>GAMGEQIFYWSPAKHWRMSDEGVVIGESTYTGMILEWFPEFYFFAQTGVTINRLLERFSSGSEKEANEILELLIQDRVLVEGILPPREVFSPQEGLFVNPYSEQIRYSKEALDYYVSEQLNRTHAACRSTKIQLETSGALPDIIQKRRSCRRFDMKTPVSFATFSNLLSSLKQRKEDKILYNYASAGGLYPIDVFVYVKPRRVEGVKAGFYYFNPADHSLVLVNNIDQVIKDDHELINQDIFAQSAFSVYLVYNARASMPKYGAAGYFYACIEAGIITATLNMVAEDLNVGLCSIGHMNFEEIQTFLKLEDHQVILHAIEGGLKIDGAAAENLYFQ[2x];> GAMEADLSEPFSLTEVQTAYMLGRNPQFELSGISPQTYFEYETELDIARLSRSFQKVIQRHPMLRAVILPEGKQQILRDVPEYEIEVESLVSMPPEKQAARLREERSRMIDHVFPLGQWPLFELKAFQLQEHTYLLCFRYDALLMDGASMNLVGQDLMHYYHQPDAQLPPLSFTFQDYMHIYDDMKRGTEYETAKAYWTNKLPDFPPAPSLLLAKDPAEIGTPNFQSLTTIITKDKWLKLRRLAQDKQVTPSALLCTVYGEVLAFWSNQRRLAINLTVFNRYPVHDEVEQIVGDFTSLILLDMDMDQKQPFFTKVEQTQSTLLDGLEHRHYDGVEFIRDYTRYHQMRPKAVMPIVFTSMLAGAGAFAWEEIGSLRHIHARTPQVYLDNVVIEKNGELLVSWNYVEELFDAEVMESMFTQFVELLDQLVEQGDINPLRISQKDYALIDQYNATAEPIPAATLHQLFIDQAQRTPDQVAVVFEQEWLTYSELDQRSNQVARFLQSRGIGRGDRVGVLAKRQVETIINLMAVLKAGAAYVPIDPDHPYERQTYILENSSCKILLDSDLYETMEISSYADGDLTPVAEPEDTAYVIYTSGSTGRPKGVIITHQAASNTIQDINRKFEVNEEDRIIGISSMCFDLSVYDIFGTLSAGATLVMIRDPRDMRELVRTVERRGITIWNTVPAIMDLALDHVGSHFENISLRLVLLSGDWIPLPLPAKINRHFPVADVISLGGATEASIWSIYWPIEQVEANWKSIPYGKPLANQTYYVLNYDQKMCPVGVIGDLYIGGAGLAQGYLNDDQKTKDAFIMHPEFGPIYKTGDCGRMRPEGYIEFLGRQDYQVKIQGYRVELEEISHCLLTYPDVDQAVVIDQTDERGMKFLVGYVVAQQEIDEKALRKHLMEHLPEYMIPAHLVHLEQLPLTPNGKLDRKALPVPKKQRNAEKFVAPQAGLEKILASVWQEVLNVEQIGANDHFFALGGDSIKAIQVSARLFVQGYHLDTKSLFEFPVLRDVARTIKKLAAAENLYFQ

The bacillamide biosynthetic pathway is a common, three-protein system, with a decarboxylase that prepares an NRPS substrate, an NRPS, and an oxidase. The oxidase is shown to perform dehydrogenation of the thiazoline in the peptide intermediate while it is covalently attached to the NRPS, as the penultimate step in bacillamide D synthesis. The oxidase forms a stable complex with the NRPS and dimerizes it. We visualized co-complexes of the oxidase bound to the elongation module of the NRPS using X-ray crystallography and cryo-EM.

The complex of BmdBM2–BmdC was subjected to structural investigation by X-ray crystallography and cryo-electron microscopy. Furthermore, though both BmdB modules of the BmdBM2-BmdC complex are visible in EM maps, the highest quality map was obtained by performing refinement with a mask that enveloped the BmdC dimer and a single BmdBM2 protomer, because the modest flexibility of the Ox:A2 interface does break the overall twofold symmetry of the full complex. Notably, the cryo-EM map was calculated using a sample in which the PCP domain was not locked into a single conformation, and as a result, the PCP and Asub domains are not visible, despite attempts at focused classification around PCP-binding sites. The EM maps do confirm the overall conformation and mode of dimerization observed by crystallography. There is some flexibility in this configuration, with the relative Ox:A2 orientation varying by ~11° across the three structures. There is clearly some flexibility visible in the EM dataset, so it is more straightforward to refine the region of the map consisting of a single BmdBM2 and a dimer of BmdC, but the BmdBM2 are in the same general orientation relative to BmdC.>GSHMATVQQLEGRWRLVDSKGFDEYMKELGVGIALRKMGAMAKPDCIITCDGKNLTIKTESTVKTTQFSCTLGEKFEETTADGRKTQTVCNFTDGALVQHQEWDGKESTITRKLKDGKLVVECVMNNVTCTRIYEKVE[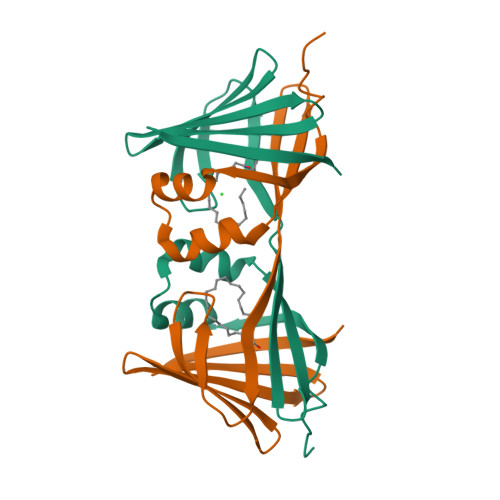2x]> PISPIETVPVKLKPGMDGPKVKQWPLTEEKIKALVEICTEMEKEGKISKIGPENPYNTPVFAIKKKDSTKWRKLVDFRELNKRTQDFWEVQLGIPHPAGLKKKKSVTVLDVGDAYFSVPLDEDFRKYTAFTIPSINNETPGIRYQYNVLPQGWKGSPAIFQSSMTKILEPFKKQNPDIVIYQYMDDLYVGSDLEIGQHRTKIEELRQHLLRWGLTTPDKKHQKEPPFLWMGYELHPDKWTVQPIVLPEKDSWTVNDIQKLVGKLNWASQIYPGIKVRQLCKLLRGTKALTEVIPLTEEAELELAENREILKEPVHGVYYDPSKDLIAEIQKQGQGQWTYQIYQEPFKNLKTGKYARMRGAHTNDVKQLTEAVQKITTESIVIWGKTPKFKLPIQKETWETWWTEYWQATWIPEWEFV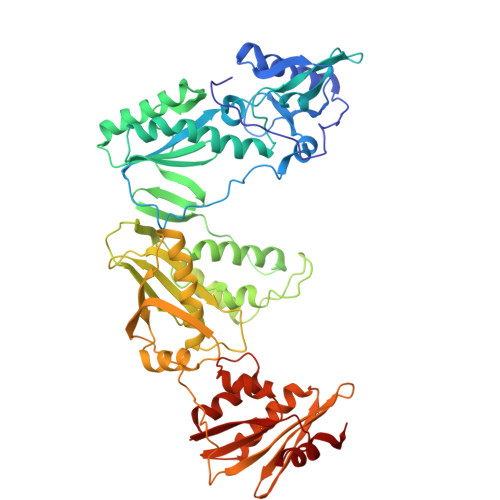NTPPLVKLWYQLEKEPIVGAETFYVDGAANRETKLGKAGYVTNKGRQKVVPLTNTTNQKTELQAIYLALQDSGLEVNIVTDSQYALGIIQAQPDKSESELVNQIIEQLIKKEKVYLAWVPAHKGIGGNEQVDKLVSAGI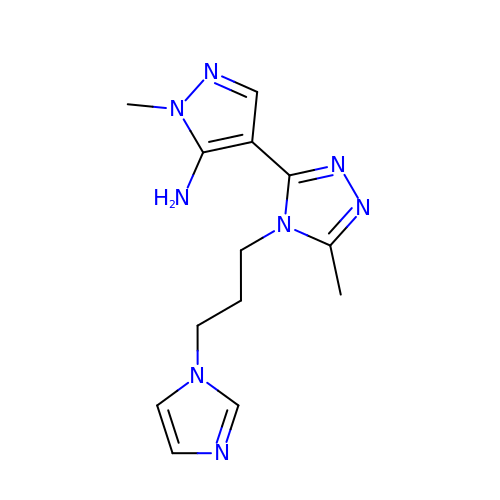4-{4-[3-(1H-imidazol-1-yl)propyl]-5-methyl-4H-1,2,4-triazol-3-yl}-1-methyl-1H-pyrazol-5-amine | C13 H18 N8 | UZDLBPIOOFFHSD-UHFFFAOYSA-N> MLRFTNCSCKTFVKSSYKLNIRRMNSSFRTETDAFGEIHVPADKYWGAQTQRSFQNFKIGGARERMPLPLVHAFGVLKKSAAIVNESLGGLDPKISKAIQQAADEVASGKLDDHFPLVV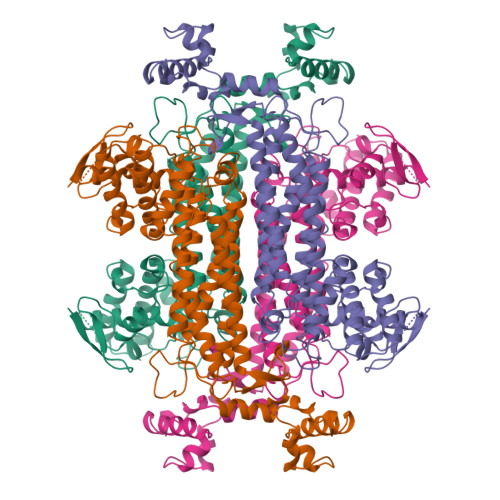FQTGSGTQSNMNANEVISNRAIEILGGKIGSKQVHPNNHCNQSQSSNDTFPTVMHIAASLQIQNELIPELTNLKNALEAKSKEFDHIVKIGRTHLQDATPLTLGQEFSGYVQQVENGIQRVAHSLKTLSFLAQGGTAVGTGLNTKPGFDVKIAEQISKETGLKFQTAPNRFEALAAHDAIVECSGALNTLACSLFKIAQDIRYLGSGPRCGYHELMLPENEPGSSIMPGKVNPTQNEALTQVCVQVMGNNAAITFAGSQGQFELNVFKPVMIANLLNSIRLITDAAYSFRVHCVEGIKANEPRIHELLTKSLMLVTALNPKIGYDAASKVAKNAHKKGITLKESALELGVLTEKEFDEWVVPEHMLGPK> MNYEEVIKKYRGEENFDHAAYDWRLHSGVTPVKDQKNCGSAWAFSSIGSVESQYAIRKNKLITLSEQELVDCSFKNYGCNGGLINNAFEDMIELGGICPDGDYPYVSDAPNLCNIDRCTEKYGIKNYLSVPDNKLKEALRFLGPISISVAVSDDFAFYKEGIFDGECGDQLNHAVMLVGFGMKEIVNPLTKKGEKHYYYIIKNSWGQQWGERGFINIETDE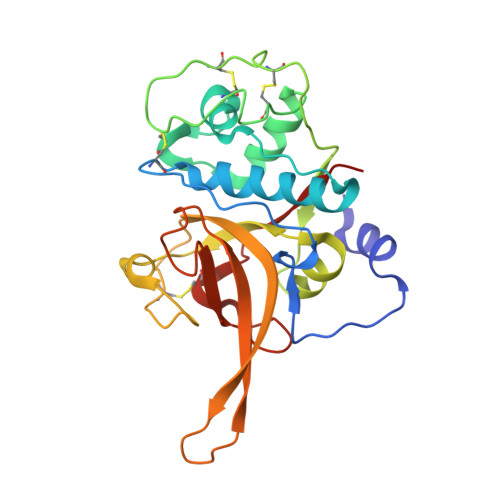SGLMRKCGLGTDAFIPLIE> GMEQEKIRIKLRAYDHRLLDQSVKQIIETVKRT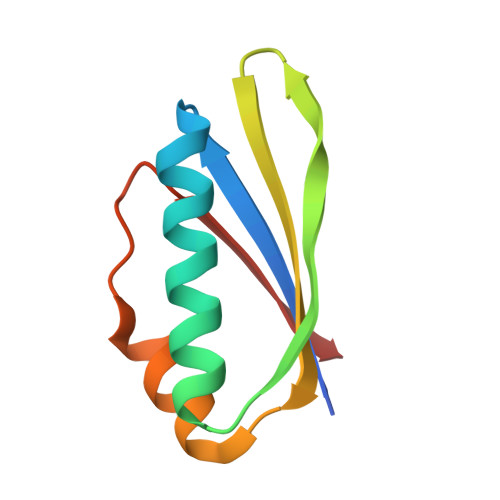GGVVKGPIPLPTRKSEFSRILDIIRFTPQTIEALMEISLPAGVDVEVKMRG> MGSWEIDPKDLTFLKELGTGQFGVVKYGKWRGQYDVAIKMIKEGSMSED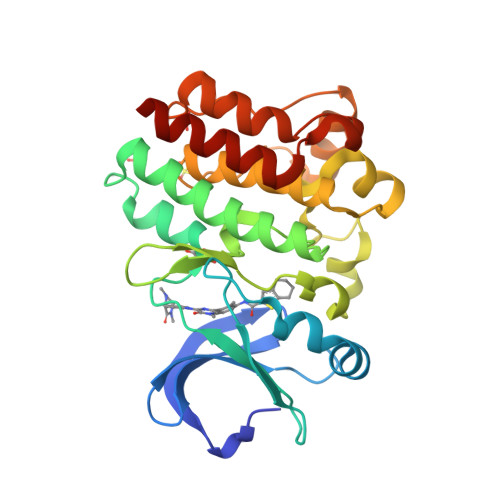EFIEEAKVMMNLSHEKLVQLYGVCTKQRPIFIITEYMANGCLLNYLREMRHRFQTQQLLEMCKDVCEAMEYLESKQFLHRDLAARNCLVNDQGVVKVSDFGLSRYVLDDEYTSSVGSKFPVRWSPPEVLMYSKFSSKSDIWAFGVLMWEIYSLGKMPYERFTNSETAEHIAQGLRLYRPHLASEKVYTIMYSCWHEKADERPTFKILLSNILDVMDENLYGN5-Se-methyl-5-seleno-alpha-D-ribofuranose | C6 H12 O4 Se | 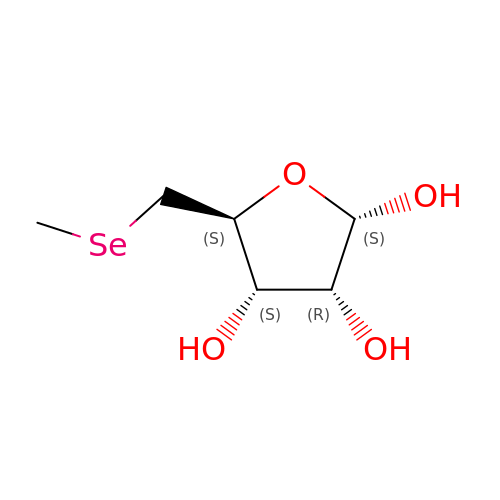UFNQFLPLDXICBS-KAZBKCHUSA-N4-[[1-(4-chlorophenyl)carbonyl-5-methoxy-2-methyl-indol-3-yl]methyl]-1,2,5-oxadiazol-3-one | C20 H16 Cl N3 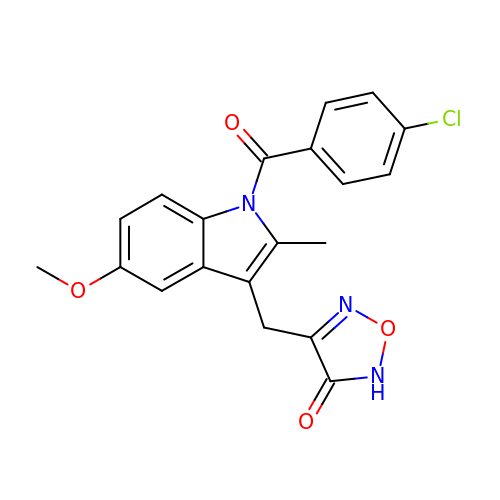O4 | VJZLOJXUWVYZRW-UHFFFAOYSA-N>[2x]FDSTDETPASYNLAVRRAAPAVVNVYNRGLNTNSHNQLEIRTLGSGVIMDQRGYIITNKHVINDADQIIVALQDGRVFEALLVGSDSLTDLAVLIIKATGGLPTIPINARRVPHIGDVVLAIGNPYNLGQTITQGIISATGRIGLNPTGRQNFLQTDASINHGNSGGALVNSLGELMGINTLSFDKSN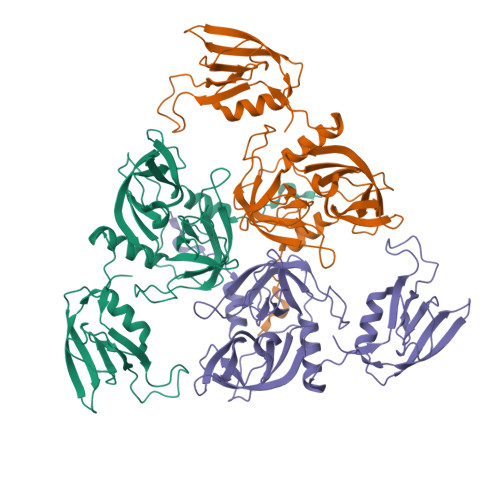DGETPEGIGFAIPFQLATKIMDKLIRDGRVIRGYIGIGGREIAPLHAQGGGIDQLQGIVVNEVSPDGPAANAGIQVNDLIISVDNKPAISALETMDQVAEIRPGSVIPVVVMRDDKQLTLQVTIQEYPAT> TGVWEKTVNTEENVYATLGSDVNLTCQTQTVGFFVQMQWSKVTNKIDLIAVYHPQYGFYCAYGRPCESLVTFTETPENGSKWTLHLRNMSSSVSGRYECMLVLYPEGIQTKIYNLLIQTHGTHHHHHH;> LEDVVVQAPTQVPGFLGDSVTLPCYLQVPNMEVTHVSQLTWA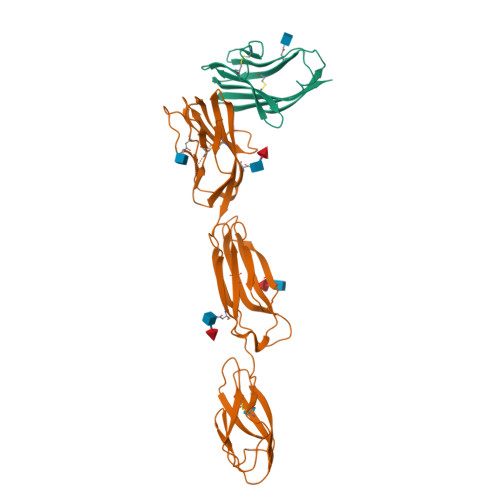RHGESGSMAVFHQTQGPSYSESKRLEFVAARLGAELRNASLRMFGLRVEDEGNYTCLFVTFPQGSRSVDIWLRVLAKPQNTAEVQKVQLTGEPVPMARCVSTGGRPPAQITWHSDLGGMPNTSQVPGFLSGTVTVTSLWILVPSSQVDGKNVTCKVEHESFEKPQLLTVNLTVYYPPEVSISGYDNNWYLGQNEATLTCDARSNPEPTGYNWSTTMGPLPPFAVAQGAQLLIRPVDKPINTTLICNVTNALGARQAELTVQVKEGPPTSHHHHHH[[(2~{R},3~{S},4~{R},5~{R})-5-(2-azanyl-6-oxidanylidene-1~{H}-purin-9-yl)-3,4-bis(oxidanyl)oxolan-2-yl]methoxy-oxidanyl-phosphoryl] [(2~{R},3~{S},4~{R},6~{R})-6-methyl-3,4-bis(oxidanyl)-5-oxidanylidene-oxan-2-yl] 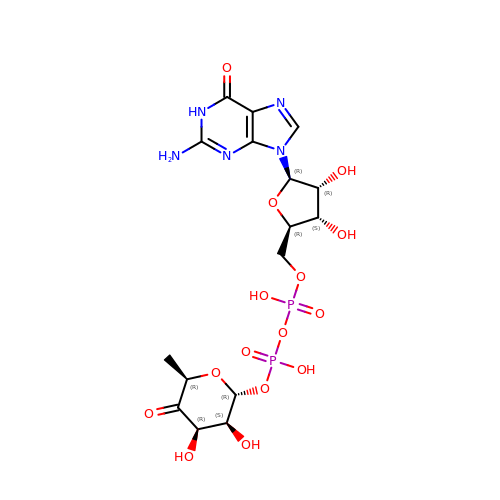hydrogen phosphate | C16 H23 N5 O15 P2 | PNHLMHWWFOPQLK-BKUUWRAGSA-N> GSSSDVVTLTVGATPSPHAKILTYINDNLAADAGIKLDIVEYTDYVQPNTALNDGDLDANFYQTVPYLENAEKQFGYNFEAGEGIHLEPLGVFSNKHKSLDELPDGGTIGIISDTANQSRALELLATQGLVSIPEGDGDVNINTVTKLKNFDFREVEGPQLVRSLDDFDYAVINGNFAQEGGKTISGDALVVESPVDNPAVNVLVWKGDSKKVDAIAKLEKLLHSD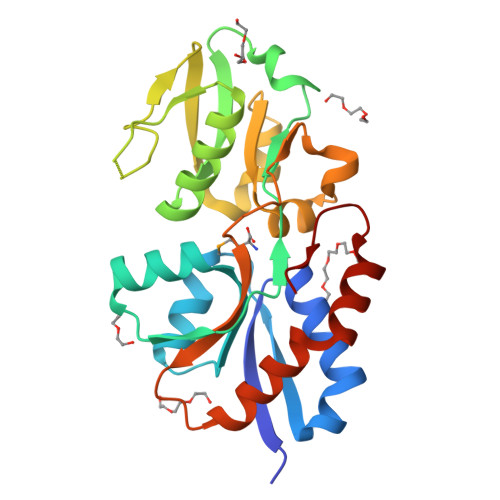EVKQYIEKTWSDGSVIPAF> GAQVSTQKTGAHETSLSAAGNSIIHYTNINYYK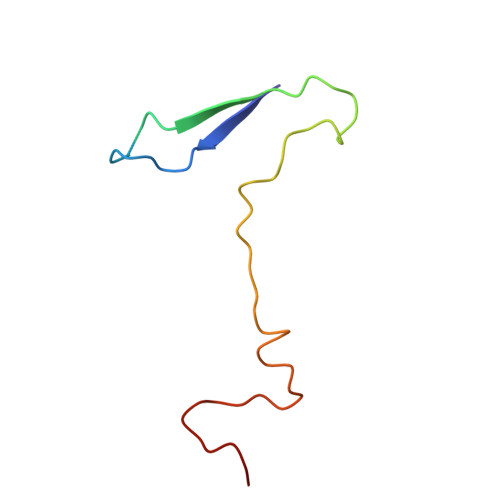DAASNSANRQDFTQDPSKFTEPVKDVMIKSLPALN> DCYH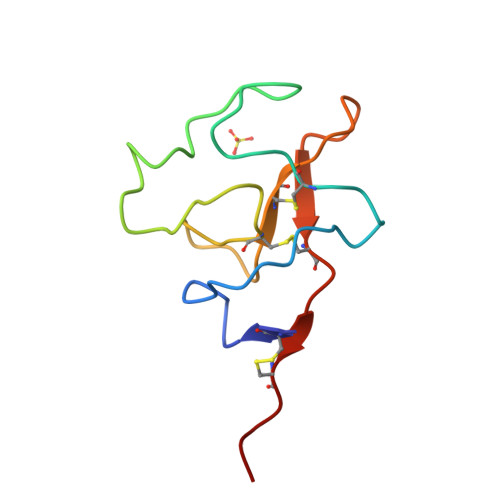GDGQSYRGSFSTTVTGRTCQSWSSMTPHWHQRTTEYYPNGGLTRNYCRNPDAEIRPWCYTMDPSVRWEYCNLTQCPVME> MSGSLSRGNGGKKVLNKNQLLKRNRIRNARSIRAEAVAASSTKTGTPSDLSESGSKLNVDQFISSRQFEVKQLQLAMHNSKAASSTRIFQALPRKLRRRTASHNVRRIPKRMRNRALREMRKSDQQDVLKGSSASSRKAHGLNAKQLYKARMSIKLLRLASKSTSMKLSMPPEVTSSNCHVRQKIKTLKRMIKESSTANPNIKLLNNRMGSYDCTGVNELAPIPKGRVKYTKRQKHFAWLPTHIWNAKRSHMMKRWGYQMVWAPTQKCFKLTHRLGGDTCSSDGALCMDSSYIGTIIVKDKSNDSEGDFLKSIIGKLTAERANLR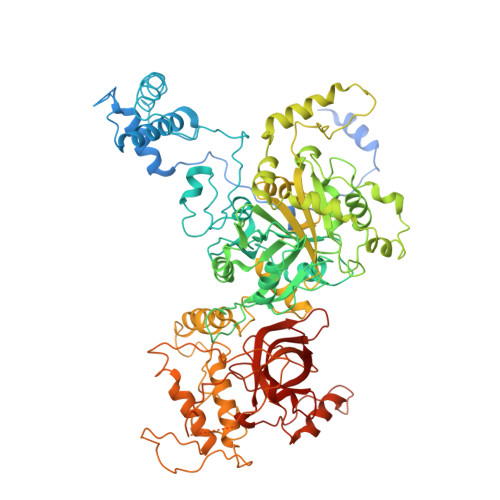KYREGQVLFQGLIYSFNEENGEDSTKPLGPCDVFWVQKDTAIIRLHPSIYTQVFNILLQHKEKLTVQDCRYSLASVTLKGAKALESLASCLRSTEYSKSFEQFKMVSMITDHNALPQRCTFAFEAIDPRHLAAPKKLNDSQRKTVNSDDILSLHENYPQDEINAVFNELCDPESRTQSYNNQNTLKEISARRYKLLTATPNSINKTTVPFKESDDPSIPLVIIRRLKTRDWIVVLPWFWLLPLWHLLNRIPRMYHIGLRQFQQIQYENKQLYFPDDYPFTQLGYIENSFYKKEASKTKWDRKPMGKRINFEKIKDIHNTKLPAYSGEIGDFFSSDWRFLQILRNGIDYLQRNDKTLELMDSKKTGQFNAQGVRDINCVNDVLEFCKDYEAKTKAMSLSIEENIPVALCKNRKCQFRTPDSISVNSSSFSLTFFPRCIIAVSCTLLERGHPKDNARIYQVPEKDLEHWLQLAKGVYRPNGRKDHDLKIPLPEVHDLIGFITSGTYHLNCGNGMGIGFIDHHAAIRQPTRYVLIRNVGTNTYRLGEWSKISV> MGEVFKEVKEKFERYKFDVVYVDREYPVS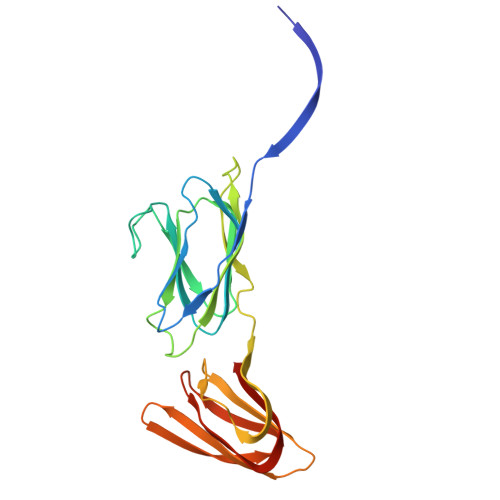SNNLNVFFEIGERNSFSGLLINEGQAVIDVLLLKKSHEGLSPIPGEGTGIQLSAGQILKFYNVPIAEIIVEYDPSNVSGVSSNVKLKGTIHPLFEVPSQISIENFQPTENYLIYSGFGTSLPQTYTIPANGYLIISITNTSTGNIGQITLTIGSTTMTFNLQTGENKIPVIAGTQITNLTLTSSSAILIYEEVI Imine reductases (IREDs) are one such enzyme class that have become widely adopted as biocatalysts for the preparation of chiral amines. These nicotinamide adenine dinucleotide phosphate‐dependent enzymes catalyze enantioselective reductions of prochiral imines to a diverse array of amine products, making them attractive targets for industrial biocatalysis. Of the enzymes tested, only one IRED sequence was identified with observable activity toward the conversion of 1 to 1a, namely, I127F L179V double mutant of IR361 (henceforth named HRED1.0) that was recently engineered by our lab for reductive amination processes involving cyclic secondary amines as substrates. Substitution of Met125 to either Phe or Trp gave substantial 6‐fold and 5‐fold increases in reaction conversion, respectively, under assay conditions used for evolution, with more modest ca. 1.5‐fold improvements observed with the H250L and A100T mutations. These beneficial mutations were subsequently combined by DNA shuffling, leading to the identification of a M125W H250L double mutant (HRED1.1) that displays a significant 20‐fold improvement in reaction conversion, and a 19‐fold improvement in reaction rate, over the parent HRED1.0 template.

The structure was determined to a resolution of 2.77 Å, with two molecules, A and B, in the asymmetric unit comprising one dimer. Two active sites are formed at the interfaces of the N‐terminal domain of one monomer and the C‐terminal bundle of the other through reciprocal domain sharing. However, the density within monomer A and the C‐terminal bundle of B was good, permitting the building of side chains and NADP+ molecule within the active site at the interface of the domains. Superimposition of the HRED1.1 structure with that of wild‐type IR361 revealed the consequences of the mutations. The substitution of I for F in position 127 at the bottom of the active site as presented in Figure 3a has, counterintuitively, made more space in the active site through the displacement of the side chain of (B)Y221. Mutation of M125 to W at the top of the active site has again created more space, despite being a larger residue as it projects upward and makes a new stabilizing interaction with the side chain of D176 through the N‐atom on the indole ring. Further stabilization of this conformation may be provided by a stacking interaction between the indole and the mutated 179 position from L to V, which lies on the interdomain helix on the other side of the active site cavity. (B)H250L is situated at the interface between the N‐terminal domain of one monomer and the C‐terminal bundle of its neighbor and may provide stabilizing hydrophobic interactions in a mode that has been observed for other IREDs in engineering studies.

>[2x]MSDPNADRPPVTVVGLGLMGQALAAAFLKGGHPTTVWNRSPEKAERLVADGAVLADTLESAVTASPLVIVCVSDYDAVHELIRPVESALAGRVLVNLTTATSTQARETAEWAAQRNIPYLDGAIWAFPPVIGTDGAVLLYSGHKSAFEAHESTLKAIAPAATTYLEEDHGLSSLYDMAVLGIMWGILNGFLHGAALLGTAKVKAETFAPLANTMISAITEYVTAYAPQVDEGRYEATDATMTVHQAAMELLAEESEHLGIHSELPRFFKTLADRAVADGHAENSYAAMIELFRKPTA(2S)-6-(2,4-DIAMINO-6-ETHYLPYRIMIDIN-5-YL)-2-(3,5-DIFLUOROPHENYL)-4-(3-METHOXYPROPYL)-2H-1,4-BENZOXAZIN-3(4H)-ONE 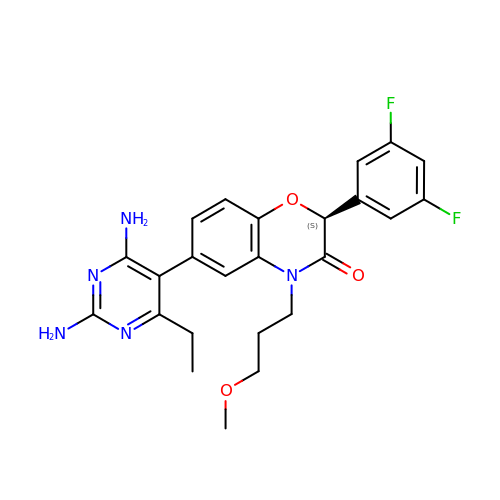| C24 H25 F2 N5 O3 | KHZQOXQOUCGGGA-NRFANRHFSA-N5-chloro-N-((1S,2R)-2-(6-fluoro-2,3-dimethylphenyl)-1-(5-oxo-4,5-dihydro-1,3,4-oxadiazol-2-yl)propyl)-4-methyl-3,4-dihydro-2H-benzo[b][1,4]oxazine-8-sulfonamide 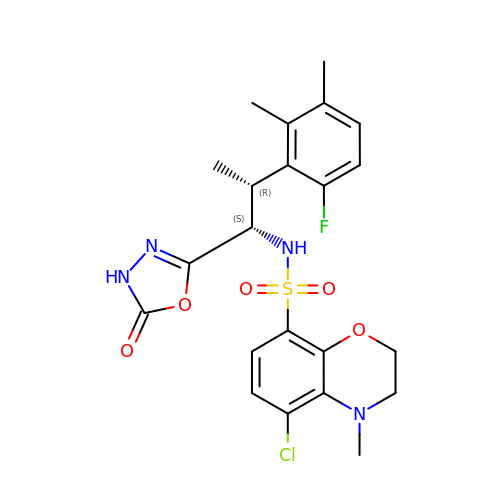| C22 H24 Cl F N4 O5 S | OODUGOCGSLORQM-ACJLOTCBSA-N> MAMSNGNNDFVVLSNSSIATSAANPSPLTPCDGDHAAQQLTPKEATRTKVSPNGCLQLNGTVKSSFLPLDNQRMPQMLPQCCHPCPYHHPLTSHSSHQECHPEAGPAAPSALASCCMQPHSEYSASLCPNHSPVYQTTCCLQPSPSFCLHHPWPDHFQHQPVQQHIANIRPSRPFKLPKSYAALIADWPVVVLGMCTMFIVVCALVGVLVPELPDFSDPLLGFEPRGTAIGQRLVTWNNMVKNTGYKATLANYPFKYADEQAKSHRDDRWSDDHYEREKREVDWNFHKDSFFCDVPSDRYSRVVFTSSGGETLWNLPAIKSMCNVDNSRIRSHPQFGDLCQRTTAASCCPSWTLGNYIAILNNRSSCQKIVERDVSHTLKLLRTCAKHYQNGTLGPDCWDMAARRKDQLKCTNVPRKCTKYNAVYQILHYLVDKDFMTPKTADYATPALKYSMLFSPTEKGESMMNIYLDNFENWNSSDGVTTITGIEFGIKHSLFQDYLLMDTVYPAIAIVIVLLVMCVYTKSMFITLMTMFAIISSLIVSYFLYRVVFHFEFFPFMNLTALIILVGIGANNAFVLCDVWNYTKFDKPHAETSETVSITLQHAALSMFVTSFTTAAAFYANYVSNITAIRCFGVYAGTAILVNYVLMVTWLPAVVVLHERYLLNIFTCFKKPQQQIYDNKSCWTVACQKCHKVLFAISEASRIFFEKVLPCIVIKFRYLWLFWFLALTVGGAYIVCINPKMKLPSLELSEFQVFRSSHPFERYDAEYKKLFMFERVHHGEELHMPITVIWGVSPEDNGNPLNPKSKGKLTLDSSFNIASPASQAWILHFCQKLRNQTFFYQTDEQDFTSCFIETFKQWMENQDCDEPALYPCCSHWSFPYKQEIFELCIKRAIMELERSTGYHLDSKTPGPRFDINDTIRAVVLEFQSTYLFTLAYEKMHQFYKEVDSWISSELSSAPEGLSNGWFVSNLEFYDLQDSLSDGTLIAMGLSVAVAFSVMLLTTWNIIISLYAIISIAGTIFVTVGSLVLLGWELNVLESVTISVAVGLSVNFAVHYGVAYRLAPDPDREGKVIFSLSRVGSAMAMAALTTFVAGAMMMPSTVLAYTQLGTFMMLIMCISWAFATFFFQCMCRCLGPQGTCGQIPLPKKLQCSAFSHALSTSPSDKGQSKTHTINAYHLDPRGPKSELEHEFYELEPLASHSCTAPEKTTYEETHICSEFFNSQAKNLGMPVHAAYNSELSKSTESDAGSALLQPPLEQHTVCHFFSLNQRCSCPDAYKHLNYGPHSCQQMGDCLCHQCSPTTSSFVQIQNGVAPLKATHQAVEGFVHPITHIHHCPCLQGRV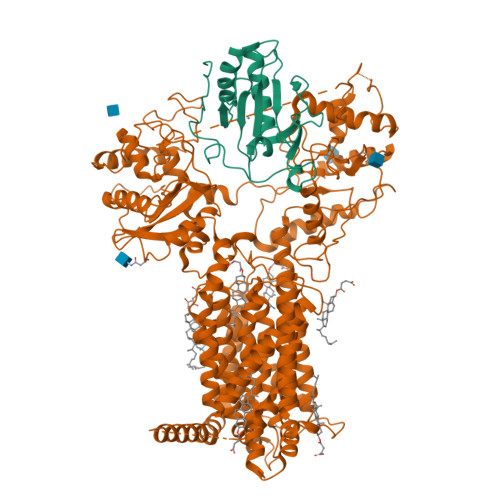KPAGMQNSLPRNFFLHPVQHIQAQEKIGKTNVHSLQRSIEEHLPKMAEPSSFVCRSTGSLLKTCCDPENKQRELCKNRDVSNLESSGGTENKAGGKVELSLSQTDASVNSEHFNQNEPKVLFNHLMGEAGCRSCPNNSQSCGRIVRVKCNSVDCQMPNMEANVPAVLTHSELSGESLLIKTL;> MLLLARCLLLVLVSSLLVCSGLACGPGRGFGKRRHPKKLTPLAYKQFIPNVAEKTLGASGRYEGKISRNSERFKELTPNYNPDIIFKDEENTGADRLMTQRCKDKLNALAISVMNQWPGVKLRVTEGWDEDGHHSEESLHYEGRAVDITTSDRDRSKYGMLARLAVEAGFDWVYYESKAHIHCSVKAENSVAAKSGGCFPGSATVHLEQGGTKLVKDLSPGDRVLAADDQGRLLYSDFLTFLDRDDGAKKVFYVIETREPRERLLLTAAHLLFVAPHNDSATGEPEASSGSGPPSGGALGPRALFASRVRPGQRVYVVAERDGDRRLLPAAVHSVTLSEEAAGAYAPLTAQGTILINRVLASCYAVIEEHSWAHRAFAPFRLAHALLAALAPARTDRGGDSGGGDRGGGGGRVALTAPGAADAPGAGATAGIHWYSQLLYQIGTWLLDSEALHPLGMAVKSS> SFESKKPMRTWSHLAEMRKKPSEYDIVSRKLHYSTNNPDSPWELSPDSPMNLWY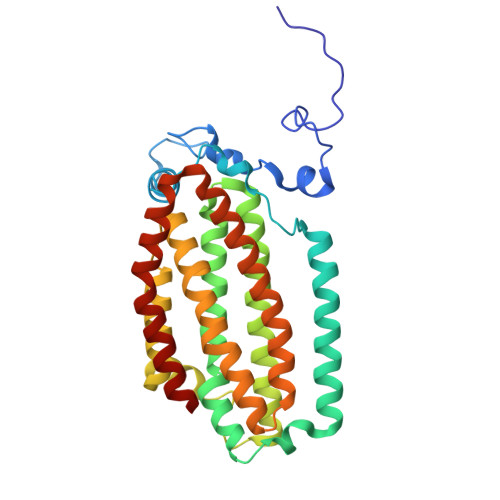KQYRNASPLKHDNWDAFTDPDQLVYRTYNLMQDGQESYVQSLFDQFNEREHDQMVREGWEHTMARCYSPLRYLFHCLQMSSAYVQQMAPASTISNCCILQTADSLRWLTHTAYRTHELSLTYPDAGLGEHERELWEKEPGWQGLRELMEKQLTAFDWGEAFVSLNLVVKPMIVESIFKPLQQQAWENNDTLLPLLIDSQLKDAERHSRWSKALVKHALENPDNHAVIEGWIEKWRPLADRAAEAYLSMLSSD> XSSD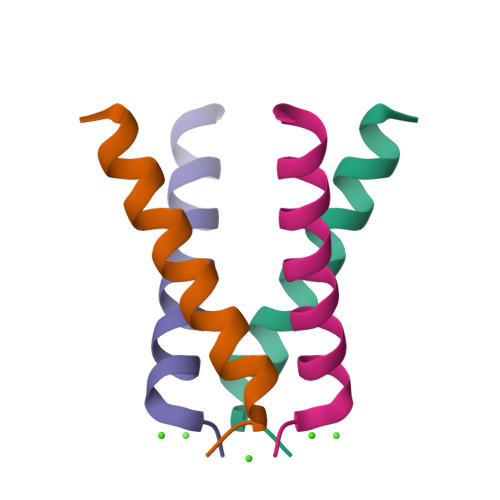PLVVAASIIGILHLILWILDRLX>MELILNEAEKVFAMHGFLGATLKQIAQNSNVTQALITYYYGTKQNLFMEVYRRGLSDIDKKRQNYLDELKSRPEGYNTYDIVRTYLRPQFEHREAGQAWMHFARLQSRLASEPEEVAVPLRKELYDHTLKAFIHEIMECEGEDDAAAVSWGAVFMVSMILYMLRGVDRIGELTDGHLHAESEDDIVERM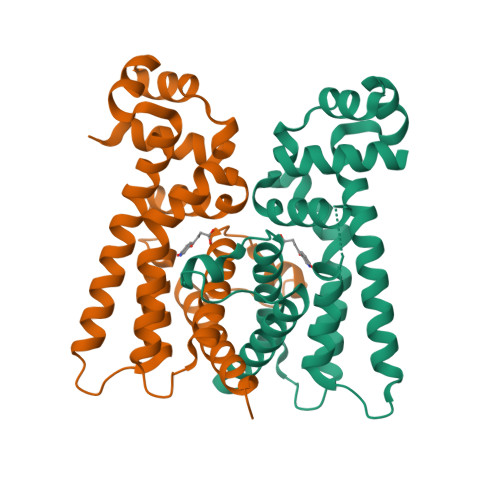TIFITGGINSLKQATQDKY[6x]>[2x]MSLLIRGATVVTHEESYRADVLCANGLIQAIGENLETPSGCDVLDGGGQYLMPGGIDPHTHMQLPFMGTVASEDFFSGTAAGL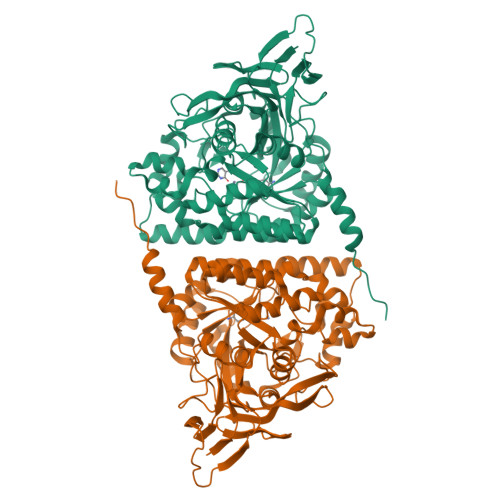AGGTTSIIDFVIPNPRQSLLEAFHTWRGWAQKSAADYGFHVAITWWSDEVAREMGELVAQHGVNSFKHFMAYKNAIMAADDTLVASFERCLELGAVPTVHAENGELVFHLQQKLLAQGLTGPEAHPLSRPPQVEGEAASRAIRIAETLGTPLYLVHISSREALDEIAYARAKGQPVYGEVLAGHLLLDDSVYRHPDWATAAGYVMSPPFRPVEHQEALWRGLQSGNLHTTATDHCCFCAEQKAMGRDDFSKIPNGTAGIEDRMALLWDAGVNSGRLSMHEFVALTSTNTAKIFNLFPRKGAIRVGADADLVLWDPQGSRTLSAATHHQRVDFNIFEGRTVRGIPSHTISQGKLLWAAGDLRAEPGAGRYVERPAYPSVYEVLGRRAERQRPVAVER>[4x]MIDLREDTWTLQLYAQRYKGLSPKNSRELQLRMEYDPLKPNLPTSGEEQNSKPEWLNTPPCLIPESESLDKAKGALVGLAIGDAIGTTLEFLPRDKLHVNDMVGGGPFRLQPGEWTDDTSMALCLAESYISAGRLDITLFREKLVRWYRHGENSSNGRCFDIGNTTRNALEQYLKHGASWFGNTEPETAGNAAIIRQAPTSIFRRKSLQRTFADSDSQSMATHCAPESMASCQFLGFILNYLINGSSREKAFSPHVMPLPVRVLLINAGEYKEKKRDEIRSSGYVIDTLEAAMWAVWNTDNFHDAILLAANLGDDADSVAATTGQIAGALYGYSNIPKPWLDKLVQQERISNLAEQLFYMAPEEDF;>HHHHHHSQDPENLYFQGQEQAKVWTQTARANAEKNNAQLSTLLTDDQIGAIYGYTTNEGYTALNPALRGQTPLTPELEAFTGHVTDGLNKLPAYNG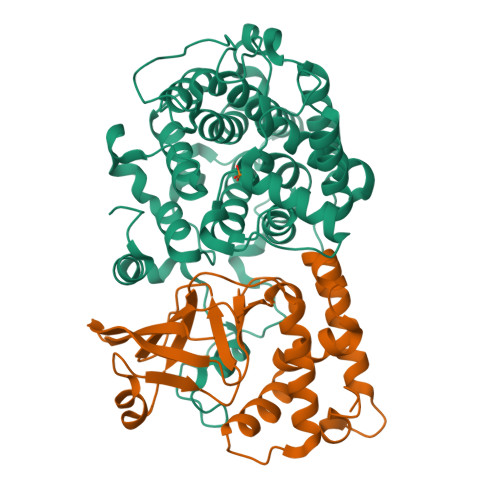ETYRGTTLPAHILEQNQIGGTVSDGGFMSTSAKTPFDGDVSISVRGNSGKQIDFLSKYKNEAEVLYPPNTRFEVINRIEQNGTTHLLYREIP[4x]>[2x]ARALQHLDPPAPLPLVIWHGMGDSCCNPLSMGAIKKMVEKKIPGIYVLSLEIGKTLMEDVENSFFLNVNSQVTTVCQALAKDPKLQQGYNAMGFSQGGQFLRAVAQRCPSPPMINLISVGGQHQGVFGLPRCPGESSHICDFIRKTLN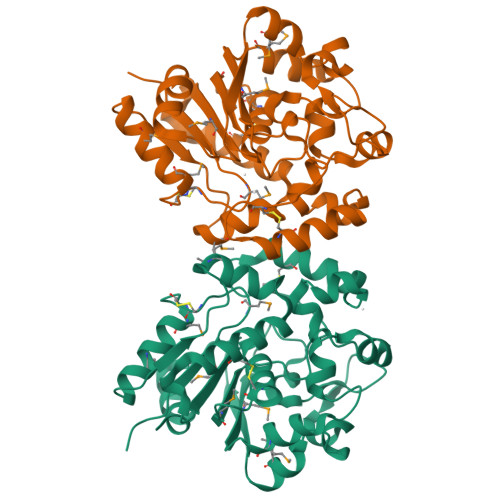AGAYSKVVQERLVQAEYWHDPIKEDVYRNHSIFLADINQERGINESYKKNLMALKKFVMVKFLNDSIVDPVDSEWFGFYRSGQAKETIPLQETSLYTQDRLGLKEMDNAGQLVFLATEGDHLQLSEEWFYAHIIPFLGEFVEHHHHHHHH> GGCUUCAUAUAAUCCGAAUGAUAUGGUUUC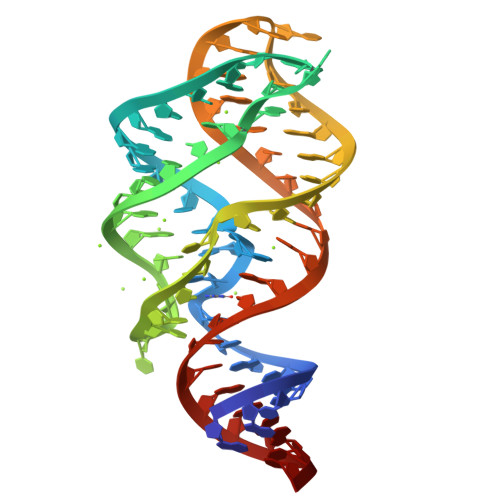GGAGCUUCCACCAAGAGCCUUAAACUCUUGACUAUGGAGUC>MVYQVKDKADLDGQLTKASGKLVVLDFFATWCGPCKMISPKLVELSTQFADNVVVLKVDVDECEDIAMEYNISSMPTFVFLKN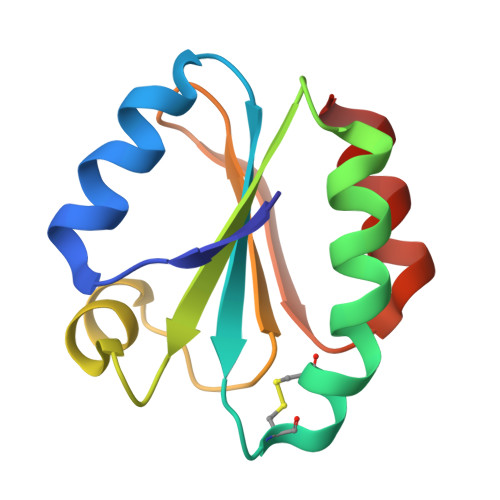GVKVEEFAGANAKRLEDVIKANI[4x]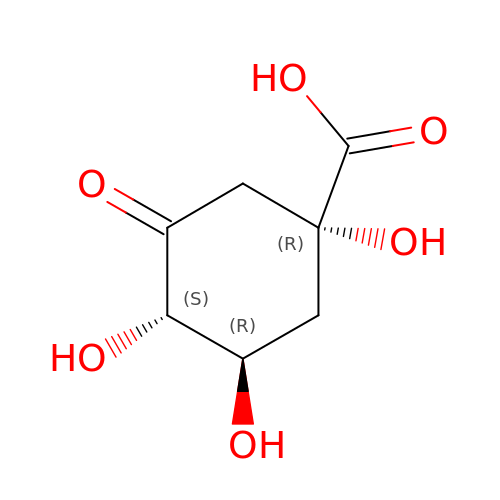1,3,4-TRIHYDROXY-5-OXO-CYCLOHEXANECARBOXYLIC ACID | C7 H10 O6 | WVMWZWGZRAXUBK-SYTVJDICSA-N Carrageenans are sulfated polysaccharides found in the cell wall of certain red algae and consist of a backbone of galactose (G) residues linked together by alternating α-1,3 and β-1,4 glycosidic bonds. Sulfatases, which remove sulfate esters, modify the functional properties of carrageenan as well as its susceptibility to various GH enzyme types. They are classified into 4 families based on sequence homology, structure and mechanism (SulfAtlas), where the S1 formyl-glycine dependent sulfatase family include most of known sulfatases. In our study, we characterized a κ-carrageenan sulfatase, AMOR_S1_16A, belonging to the sulfatase S1_16 subfamily, which selectively desulfates the nonreducing end galactoses of κ-carrageenan oligomers in an exomode.

Here, we describe the identification, production and functional – and structural characterization of a thermostable carrageenan sulfatase identified from a metagenomic data set collected from the Arctic Mid-Ocean Ridges (AMOR). Named AMOR_S1_16A, this enzyme exhibits an exoacting mechanism, removing the sulfate ester at position 4 of the nonreducing end of κ-carrageenan oligomers. AMOR_S1_16A represents the first identified and structurally solved κ-carrageenan sulfatase from the S1_16 subfamily. With only a limited number of available structures, it introduces an important novel functionality to the diverse and complex enzyme repertoire for carrageenan processing, while enhancing our understanding of the substrate specificity and characteristics of the S1_16 subfamily. S1 sulfatases are calcium-dependent and contain an essential calcium binding site (typically D-D-D-Q/N) conserved across all S1 sulfatases with known 3D structure. They require post-translational modification of a cysteine or serine to formyl-glycine, which is catalyzed by the formyl-glycine generating enzyme. Additionally, S1 sulfatases share a set of polar residues in the catalytic site crucial for sulfate hydrolysis.

> MGAQRPPDKLNFIIILIDDYGWTDSTCYGSTFYETPNIDRLAREGMRFTNAYAACPVCSPTRASILTGKYPAHLHLTDWIPGRKQWPTSKLLGAPFYQELPLWETTIAERLKPLGYTTAAMGKWHLGHEPYYPERQGFDINVAGTFRGHPESYFGPFDLPNFRGWTKNDYLTDRLTDKALQFLEENRQRPFFLYLAHFAVHTPLQAKAEMIAKYERKARGRKLQKNPTYAAMIESMDQGVGRVMSKLEDLKIADHTVIIFTSDNGGLMYEGSRREPVTSNRPLRAGKGHLYEGGVRVPLIIRWPGVVKPGTTCDVPACSVDFFPTIEEMAGLRHDPKLALDGVSLTPLLRRKGGFKPRALYWHYPHYSNQGGVPGGAIREGNLKLIEFYEDSHVELYDLSEDIGERHNLAKEMPDKAAELQAKLKAWRASVRATMPTVNPNYDPARADQGLTGADPAHQLEHHHHHH>LPISMSDEGDSFLVKDSLGENKIPKNPSKVVILDLGILDTFDALKLNDKVVGVPAKNLPKYLQQFKNKPSVGGVQQVDFEAINALKPDLIIISGRQSKFYDKLKEIAPTLFVGLDNANFLSSFENNVLSVAKLYGLEKEALEKISDIKNEIEKAKSIVDEDKKALIILTNSNKISAFGPQSRFGIIHDVLGINAVDENIKVGTHGKSINSEFILEKNPDYIFVVDRNVILGNKERAQGILDNALVAKTKAAQNKKIIYLDPEYWYLASGNGLESLKTMILEIKNAVK[2x]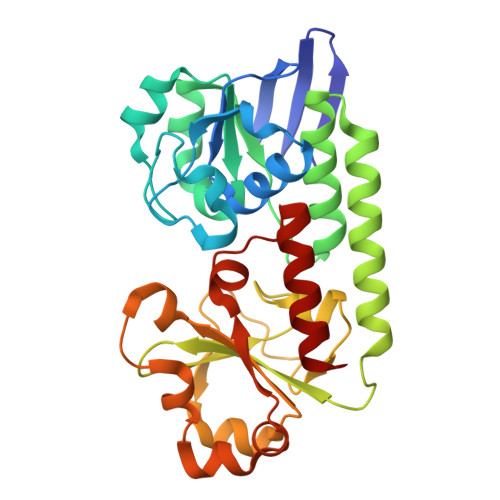;> IPISMSDEGDSFLVKDSIGENKIPKNPSKVVILDLGILDTFDALKLNDKVVGVPAKNLPKYLQQFKNKPSVGGVQQVDFEAINALKPDLIIISGRQSKFYDKLKEIAPTLFVGLDNANFLSSFENNVLSVAKLYGLEKEALEKISDIKNEIEKAKSIVDEDKKALIILTNSNKISAFGPQSRFGIIHDVLGINAVDENIKVGTHGKSINSEFILEKNPDYIFVVDRNVILGNKERAQGILDNALVAKTKAAQNKKIIYLDPEYWYLASGNGLESLKTMILEIKNAVK>CGRTSCHLPRDVLTRACAYQDRRGQQRLPEWRDPDKYCPSYNKSPQSNSPVLLSRLHFEKDADSSERIIAPMRWGLVPSWFKESDPSKLQFN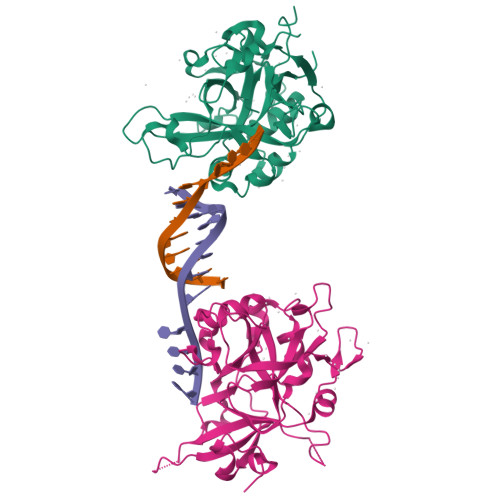TTNCRSDTVMEKRSFKVPLGKGRRCVVLADGFYEWQRCQGTNQRQPYFIYFPQIKTEKSGSIGAADSPENWEKVWDNWRLLTMAGIFDCWEPPEGGDVLYSYTIITVDSCKGLSDIHHRMPAILDGEEAVSKWLDFGEVSTQEALKLIHPTENITFHAVSSVVNNSRNNTPECLAPVAENLYFQ[2x]>[2x]GHMHPPNRRGISFEVGAQLEARDRLKNWYPAHIEDIDYE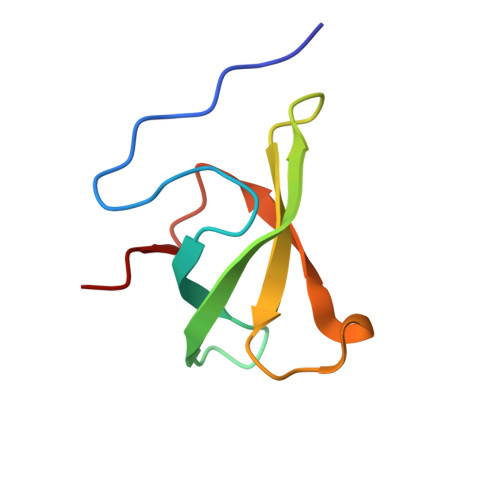EGKVLIHFKRWNHRYDEWFCWDSPYLRPLE KIF20A is a critical kinesin for cell division and a promising anti-cancer drug target. Among these, the Kin-6 KIF20A (MKLP2, Rabkinesin-6) plays critical roles during the metaphase/anaphase transition and cytokinesis. Among the kinesin classes, Kin-6 motor domains are unique in having long N- and C-terminal extensions as well as a particular long sequence inserted within loop L6. We also provide, for the first time, a detailed description of unique sequence differences and their consequences for the structure and function of this atypical kinesin by solving high resolution structures of the nucleotide-free (NF) state of KIF20A, bound and unbound to a microtubule, using cryo-electron microscopy (cryo-EM) and X-ray diffraction, respectively.

We obtained a 2.7 Å resolution structure of a microtubule-unbound murine KIF20A fragment (residues 55–510) comprising the MD and the first residues of the NL. Overall, the MD structure displays a typical kinesin fold with the MD in the open conformation, which is generally not observed for isolated kinesins. Instead, this open conformation is one of the conformations observed when kinesins are bound to a microtubule or tubulin. Close to the P-loop, a sulfate ion is found at the position normally occupied by the nucleotide β-phosphate. (c) The open NBS of KIF20A MD alone (X-ray structure) showing disordered switch loops. The difference is due to a bias in the β6-L10-β7 conformation in the X-ray structure that is involved in crystal packing contacts. The common interactions between L6-N and MD core residues are particularly well defined in the crystal structure, showing multiple hydrophobic contacts, especially in the βL6-βL6′ region (bottom). We also found that addition of 5–10 mM Mg2+·ADP did not disrupt the possibility to crystallize KIF20A in the same conformation. No nucleotide density or ordering of the NBS was visible in the electron density maps in this case. No ADP was visible in the nucleotide binding site of the resulting model, which was thus refined against another native crystal dataset obtained in nucleotide-free conditions.

> MALLEDTSEKVKVYLRIRPFLTSELDRQEDQGCVCIENTETLVLQAPKDSFALKSNERGVGQATHKFTFSQIFGPEVGQVAFFNLTMKEMVKDVLKGQNWLIYTYGVTNSGKTYTIQGTSKDAGILPQSLALIFNSLQGQLHPTPDLKPLLSNEVIWLDSKQIRQEEMKKLSLLIGGLQEEELSTSVKKRVHTESRIGASNSFDSGVAGLSSTSQFTSSSQLDETSQLWAQPDTVPVSVPADIRFSVWISFFEIYNELLYDLLEPPSHQHKRQTLRLCEDQNGNPYVKDLNWIHVRDVEEAWKLLKVGRKNQSFASTHMNQQSSRSHSIFSIRILHLQGEGDIVPKISELSLCDLAGSERCKHQKSGERLKEAGNINTSLHTLGRCIAALRQNQQNRSKQNLIPFRDSKLTRVFQGFFTGRGRSCMIVNVNPCASTYDETLHAAKFSALASQLVHAPLEHHHHHH> MGSSHHHHHHSSGETVRFQGHMRNPAMYSEEARLKSFQNWP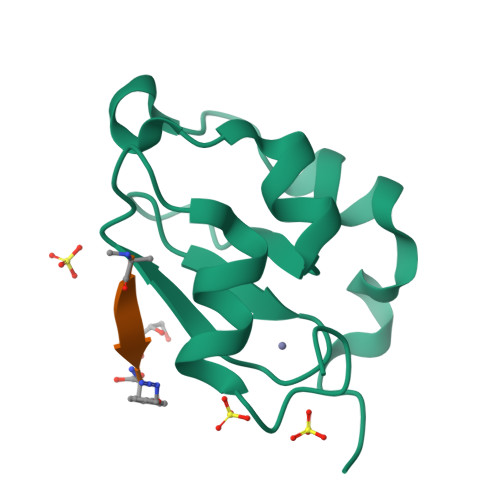DYAHLTPRELASAGLYYTGIGDQVQCFACGGKLKNWEPGDRAWSEHRRHFPNCFFVL> MGSDKIHHHHHHKGKIQEADNAAKLSAIKFVLKDPLTGDYLVDEKEIEEIVKKTGIETVVLKEYKEGVVLGPLYEFVTKDGRNAYVLSGYAPGFGGNVTVVACFIKTEDGFMLNSVRVIDYSQETPG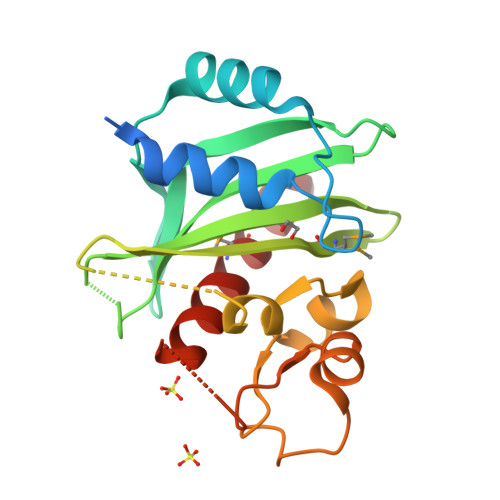LGAKIGEESIQRRFFPVPPEGLKNGLRVDKDAGLPKGSPEELKKQGIVKVSDVMTGATITPRAVVTALNLMYRYLEEVSK> SAGAEPAPEPRRFTIEVNGRRFGVAVFGDGMNATPVASPSRSAPARRAAPKKTTLAAPVDAVISPIQGRVVAVRVAHGQQVEAGQVLFIVEAMKMENEITA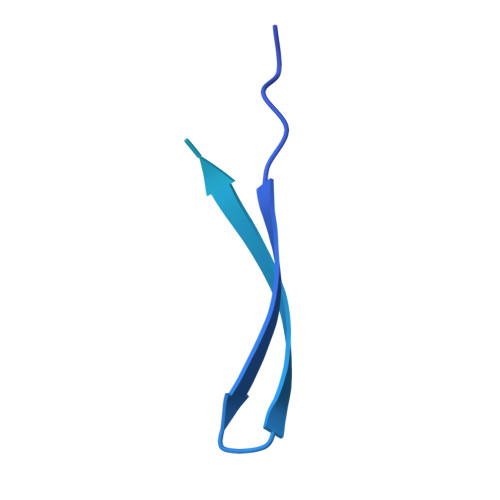PHSGTIAEVRVEVGTTVEAGAMLATYQNTANNTNGK> MLSAHQWLRHCIIGVASVALLQACSKQTGNESSSSAKSATEQVKALAQVERTAEGVVLTLPEGTVKKLRLQVMGERIIRVTALPGTDFGIVPESIQVVAKPATNVPFSVDQAGEKLVLKTSQVSAEVSLLDGTVSFRDAKGNVLLQEENRGTFSPVIHDPDPVDADSYALRQEFNRGSDEGFFGLGQHQNGQVNYAGENVELTTYNLVISIPFLVSSRNYGLLWDNNSITRFGDPREAQPLNQSLKLYDAEGKEGGLTVRYFVGDELKLTRVEADFNHQFYKQGNELENPFPEEVAGAYKNNTLRIELEGSIEAQATGKHQFKMYNSGYAQLSLDGEVVLDRWRMNWNPWYHNFYRELNAGDKHKLKVSWKPDGGFFHLRHLDPLPANEQHELSLASETGKAIDYYFVAGDTKDDIISGYRQLTGKSVMLPKWAYGFWQSRERYKSSDEIIQNLKEYRDRKIPIDNIVLDWSYWPEDAWGSHDF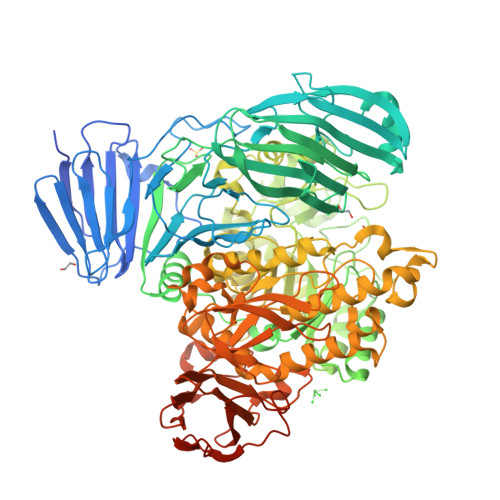DKQFFPDPKALVDKVHAMNAQIMISVWPKFYPTTDNYKELNAKGFMFNRNLDEKNLDWIGKGYLNAFYDPFSPEATAIFWKQIRDKINVHGFDAWWLDAVEPDIHSNLTFEKRKWLMTPNARGNGAEIFNAYAVPHAEGVYQGELATDGDKRSFILTRSGFGGIQRTGSAIWSGDIVSRWSDMKDQIAAGIGTNLAGVTNWTFDIGGFTPEDRFRHGKKGFVGSWTALDAEQVDEWQELNTRWYQFGAFVPLYRSHGQNPYREIFNIADEGTEVYNAMVWYTKLRYYLMPYIYTLGGDTYHKDGTIMRGLVMDFPNDRKAWDINTQYMFGPAFLVNPVYEYKARSRDVYLPAGSDWYNFYTGEKLAGGQTITADAPLARVPLFVKAGAIVPTGPLIQHVDEGLNSPLLITVYTGANGSFDIYEDDGRSLKYQQGEWSRIPLSYDDVTGTLIIGDRVGSFTGMADERNIRVRFIAGPTADATNFDKAAAEAVTYTGKSVSIKRPRKVVINSKLEGKPIPNPLLGLDSTRTGHHHHHH> DFI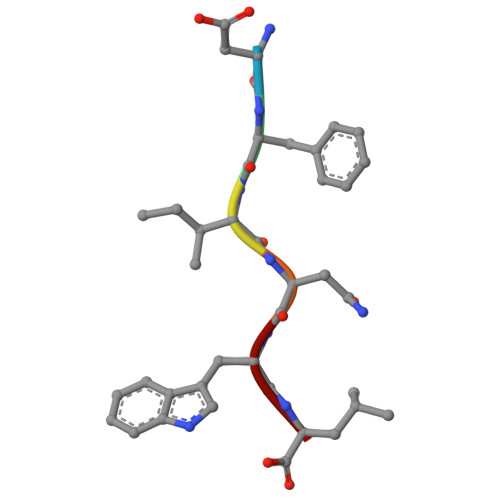NWL> DYKDDDDKGGGGSFRDCADVYQAGFNKSGIYTIYINNMPEPKKVFCNMDVNGGGWTVIQHREDGSLDFQRG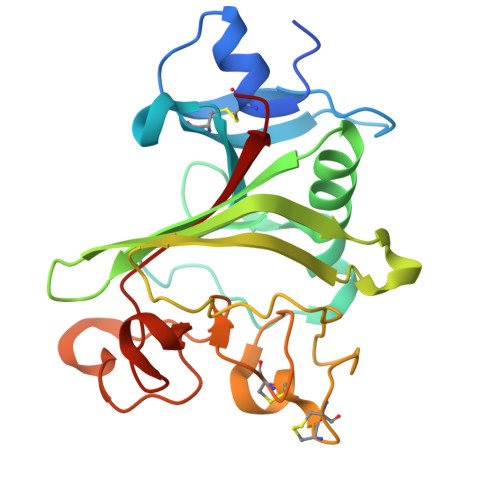WKEYKMGFGNPSGEYWLGNEFIFAITSQRQYMLRIELMDWEGNRAYSQYDRFHIGNEKQNYRLYLKGHTGTAGKQSSLILHGADFSTKDADNDNCMCKCALMLTGGWWFDDCGPSNLNGMFYTAGQNHGKLNGIKWHYFKGPSYSLRSTTMMIRPLDF> PKALIVYGSTTGNTEYTAETIARELADAG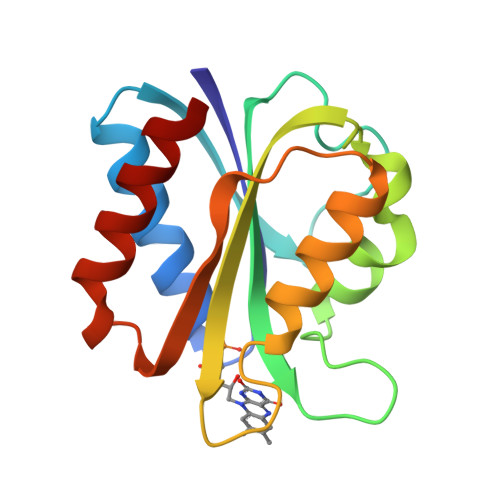YEVDSRDAASVEAGGLFEGFDLVLLGCSTWVDDSIELQDDFIPLFDSLEETGAQGRKVACFGCGDSSYEYFCGAVDAIEEKLKNLGAEIVQDGLRIDGDPRAARDDIVGWAHDVRGAI> PISPIETVPVKLKPGMDGPKVKQWPLTEEKIKALVEICTEMEKEGKISKIGPENPYNTPVFAIKKKDSTKWRKLVDFRELNKRTQDFWEVQLGIPHPAGLKKKKSVTVLDVGDAYFSVPLDEDFRKYTAFTIPSINNETPGIRYQYNVLPQGWKGSPAIFQSSMTKILEPFRKQNPDIVIYQYMDDLYVGSDLEIGQHRTKIEELRQHLLRWGLTTPDKKHQKEPPFLWMGYELHPDKWTVQPIVLPEKDSWTVNDIQKLVGKLNWASQIYPGIKVRQLSKLLRGTKALTEVIPLTEEAELELAENREILKEPVHGVYYDPSKDLIAEIQKQGQGQWTYQIYQEPFKNLKTGKYARMRGAHTNDVKQLTEAVQKITTESIVIWGKTPKFKLPIQKETWETWWTEYWQATWIPEWEFVNTPPL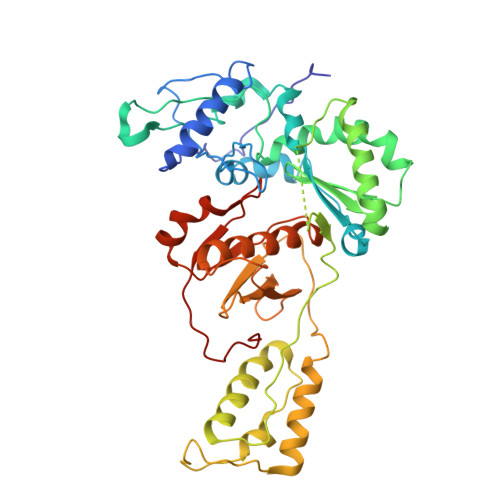VKLWYQLGGHHHHHH> VTNVGEDGEPGETEPRHALSPVDMHVHTDVSFLLDRFFDVETLELSNLTGSPATHVLDPFGSTAQLAWARLLNTCTYFFSDLELSIQFKFTTTPSSVGEGFVWVKWFPVGAPTKTTDAWQLEGGGNSVRIQQLAVAGMSPTVVFKIAGSRSQACGFSVPYTSMWRVVPVFYNGWGAPTKEKATYNWLPGAHFGSILLTSDAHDKGGCYLRYRFPRANMYCPRPIPPAFTRPADKTRHKFPTNINKQ;> DKKTEETTNIEDRIETTVVGATIINSQGSVGTTYCYSKPDGRPPSTVSDPVTRLGPTLSRHYTFKVGEWPHSQSHGHAWICPLPSDKLKKMGSFHEVVKAHHLVKNGWDVVVQVNASFAHSGALCVAAVPEYEHTHEKALKWSELEEPAYTYQQLSVFPHQLLNLRTNSSVHLVMPYIGPGPTTNLTLHNPWTIVILILSELTGPGQTVPVTMSVAPIDAMVNGPLPNPE;> APIRVVSVPESDSFMSSVPDNSTPLYPKVVVPPRQVPGRFTNFIDVAKQTYSFCSISGKPYFEVTNTSGDEPLFQMDVSLSAAELHGTYVASLSSFFAQYRGSLNFNFIFTGAAA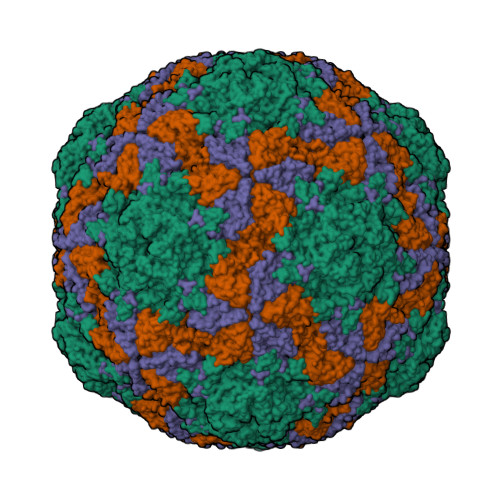TKAKFLVAFVPPHSAAPKTRDEAMACIHAVWDVGLNSAFSFNVPYSSPADFMAVYSAEATVVNVSGWLQVYALTALTSTDIAVNSKGRVLVAVSAGPDFSLRHPVDLPDKQ;> GAGTSTPTTGNQNMSGNSGSIVQNFYMQQYQNSIDADLGDNVISPEGQGSNTSSSTSSSQSSGLGGWFSSLLNLGTKLLA> LNCGQVDSKMKPCLTYVQGGPGPSGECCNGVRDLHNQAQSSGDRQTVCNCLKGIARGIHNLNLNNAASI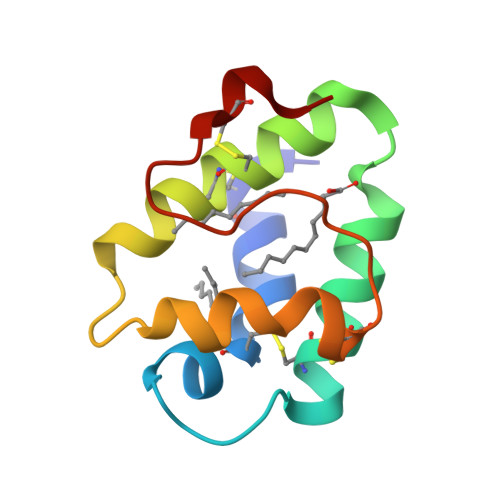PSKCNVNVPYTISPDIDCSRIY> GSTDLFSSPDHTLDALGLRCPEPVMMVRKTVRNMQPGETLLIIADDPATT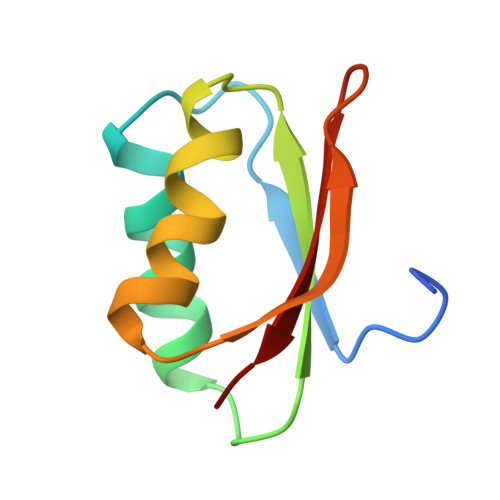RDIPGFCTFMEHELVAKETDGLPYRYLIRKGG1-[[3-[3,5-bis(chloranyl)phenyl]-5-[(4-pyridin-4-ylpiperazin-1-yl)methyl]phenyl]methyl]-4-pyridin-4-yl-piperazine | 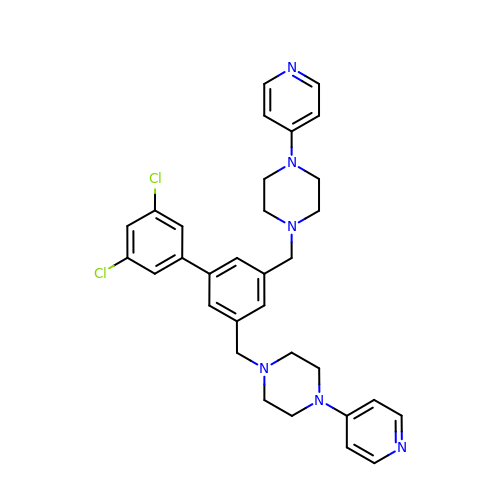C32 H34 Cl2 N6 | IFPHOKXTHCEYJO-UHFFFAOYSA-N> MSARGRAAGDDGRQAELMATLGFVRLSKSSVGKVKKFLNNLYDLKSINLCRHPRVIAECRGTDLSRETQLYNEMVLWLRYHEKLTARRPGHLPLLTRIRQDYDKLFGFVAARPELCGFDGLTEVNVFDDAVYGDDYVPRVDVFLRGLEDLARCLCAQGPDKPARAVIMGFINMRAEEVNRLMDNVRDAAERVLVYEVLDVRDPLNEDPSVLVHNRLVYLCRLAYAISKSWQTLSHMCLDRINSLRRRLILAFHDRPAFARVYARNALERPVDGTTAYNLLRRLEEDFLLFRNALRWGDPDWGLESELESEGDNSDAGSDLDLEDEEDDDDGGGPGGHDDESGGNRTPDPGMSLHDDTGIANTCLIGGDDEDCGGGSGRCLEFDPDSERCLGVKMVNGRALRWWNPTGIMVDNEAAVWIDEHGRVMDKPPPKELRKASSDD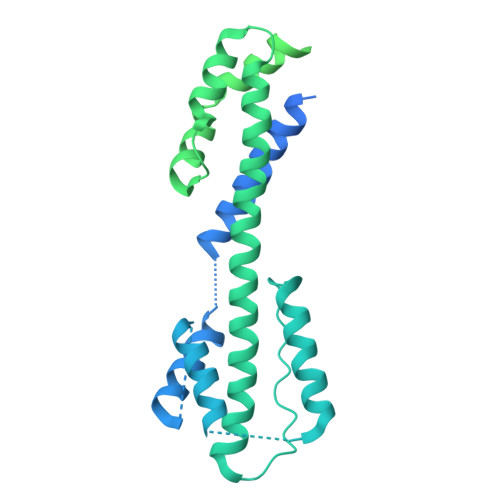GGNKKNPPPKKNVTPPVSGSNSVGGGVQTPSTASGKRTGKKKEGGGGYLLRSRSTDDDEVRKMKKDGTIDDRADRELKMALQKARESTADSDLSTILPRTEPLRKVAFVGDPVAAFGDTVRTTSSSKGFDDGPFTTQGASVLLPPPLGGPGSTLTLPPDLPDLSGVLADEDVQDSRYGKIPKSRTKKHPTFPENYKQRPPPHNKDDEYYWDETGDNMPVGEDGGGVLEDLRKGLEGIDLKTGGGGSLQPPLSQQFAGSPFAGSDGDGGGLVKKSSSSH> MGMVVALGLAFGTSGARAIACDFDSDRSVSVSVTFPKTSQNWPQVWREALWQLLTQIPADWRSRIERIAIDGTSGTVLLCDREGQPQTEPLLYNQACPIDLADLADWVPADHAALSSTSSLAKLWFWQQQFGALPPDWQILAQADWLSLQLHGCSQQSDYHNALKLGYSPDRERFSKNLLDSE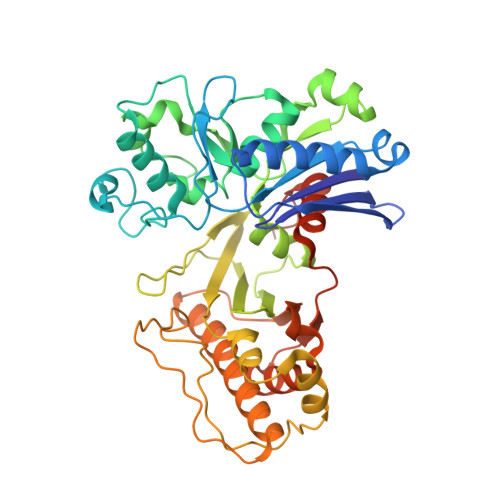LGALLPVVHEPGVAIGPILPAIAQEFGLSPDCQICAGTTDSIAAFLASGAHQPGEAVTSLGSTIVLKLLSQVAVSDRLTGVYSHKLGGYWLTGGASNCGGATLRQFFPDTELESLSCQIDPTKKSGLDYYPLPSRGERFPIADPDRLPQLEPRPENPVQFLQGLLEGLTQVETLGYQRLQDLGATPLKRIWTAGGGAKNAVWQQLRQQAIGVPIAIAPNTEAAFGTARLAAFGLAAFHSAGLKRTLEHHHHHH Cytoplasmic incompatibility (CI) results when Wolbachia bacteria-infected male insects mate with uninfected females, leading to embryonic lethality. CI is caused by linked pairs of Wolbachia genes called CI factors (CifA and CifB). Protein-binding experiments and expression of cif genes in yeast have shown that CifA binds its cognate CifB specifically and rescues CifB-induced yeast growth defects. CidBwMel consists of a region, which is predicted to contain two PD-(D/E)XK (pseudo) nuclease domains (residue 1-751; hereafter CidBwMelND1-ND2, ND: nuclease domain) and a C-terminal deubiquitylase (DUB) domain.

We determined the crystal structure of the CidBwMel DUB domain to 1.85 Å resolution. Similar to the structures of other proteases in the CE clan/Ulp1-like protease family, the DUB core consists of a five-stranded β sheet flanked by α helices on both sides. His957, Asp976, and Cys1016 form the catalytic triad. An active DUB domain is required for inducing a CI-like phenotype in transgenic D. melanogaster for cid operons. The crystal structure of CidBwMelDUB provides a solid structural basis for further investigation of the molecular targets and function of CidB deubiquitylase family proteins. Given that bacteria do not possess a ubiquitin-conjugation system, the presence of a DUB domain in CidB strongly suggests that this Wolbachia protein functions within the host.

> GPLGSGTSTAQGILQQINTILRRNNAREIEDVHNLLALDFATENQNFRYWLQTHDMFFAARQYTFHDDRSNPTNDRHDFAITSVGVDGNQNDPTGRDLLSSNIDNFKQKVDSGEKDRLTAIINVGNRHWVTLVIVHQNGNYYGYYADSLGPDSRIDNNIRGALRECDISDDNVHDVSVHQQTDGHNCGIWAYENARDINQAIDQALQGNSNFGEKGEGIIGYIRGLLSAGIGNDTRQPQRNEQYFRNRRRNISQLFQNDSLSSPRGRLIQGRPGIQHEIDPLLLQFLELQYPQ3-(dimethyl-lambda~4~-sulfanyl)propanoic acid | C5 H12 O2 S | 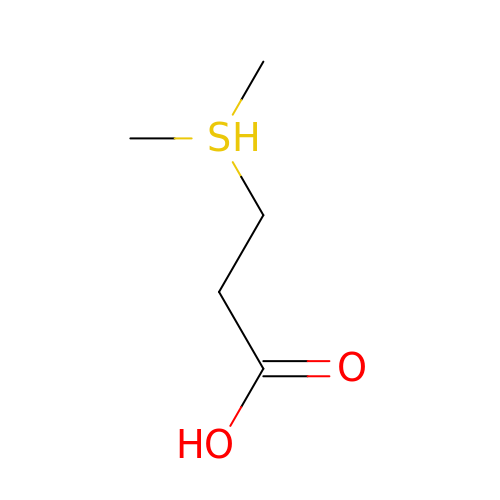BBSYGEAKHYDEGI-UHFFFAOYSA-N N-[(2S)-1-[4-(5-BROMOPYRIDIN-2-YL)PIPERAZIN-1-YL]SULFONYL-5-PYRIMIDIN-2-YL-PENTAN-2-YL]-N-HYDROXY-METHANAMIDE | C19 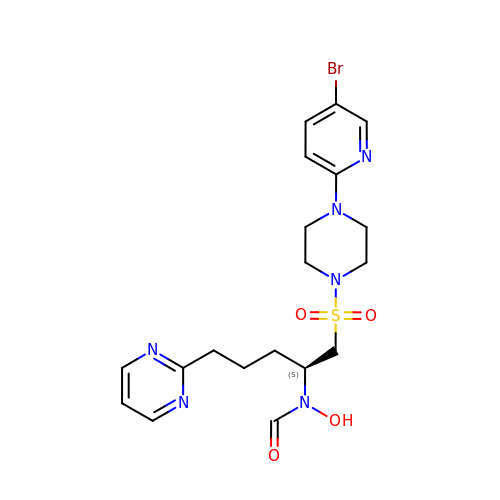H25 Br N6 O4 S | KOKUKBSLFSEGAT-KRWDZBQOSA-N>MPEITESERAYHLRKMKTRMQ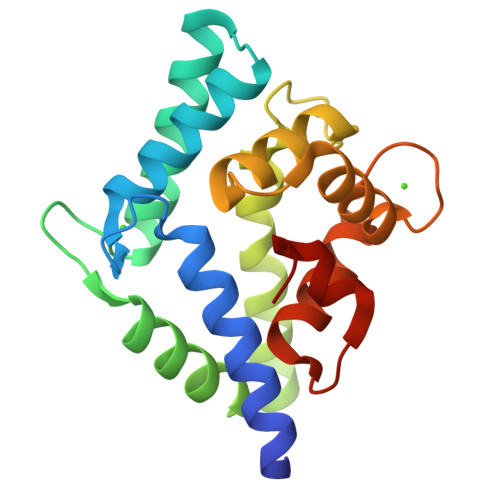RVDVTGDGFISREDYELIAVRIAKIAKLSAEKAEETRQEFLRVADQLGLAPGVRISVEEAAVNATDSLLKMKGEEKAMAVIQSLIMYDCIDTDKDGYVSLPEFKAFLQAVGPDLTDDKAITCFNTLDFNKNGQISRDEFLVTVNDFLFGLEETALANAFYGDLVD[2x]> SYHKPDQQKLQALKDTANRLRISSIQATTAAGSGHPTSCCSAAEIMAVLFFHTMRYKSQDPRNPHNDRFVLSKGHAAPILYAVWAEAGFLAEAELLNLRKISSDLDGHPVPKQAFTDVATGSLGQGLGAACGMAYTGKYFDKASYRVYCLLGDGELSEGSVWEAMAFASIYKLDNLVAILDINRLGQSDPAPLQHQMDIYQKRCEAFGWHAIIVDGHSVEELCKAFGQAKHQPTAIIAKTFKGRGITGVEDKESWHGKPLPKNMAEQIIQEIYSQIQSKKKILATPPQEDAPSVDIANIRMPSLPSYKVGDKIATRKAYGQALAKLGHASDRIIALDGDTKNSTFSEIFKKEHPDRFIECYIAEQNMVSIAVGCATRNRTVPFCSTFAAFFTRAFDQIRMAAISESNINLCGSHCGVSIGEDGPSQMALEDLAMFRSVPTSTVFYPSDGVATEKAVELAANTKGICFIRTSRPENAIIYNNNEDFQVGQAKVVLKSKDDQVTVIGAGVTLHEALAAAELLKKEKINIRVLDPFTIKPLDRKLILDSARATKGRILT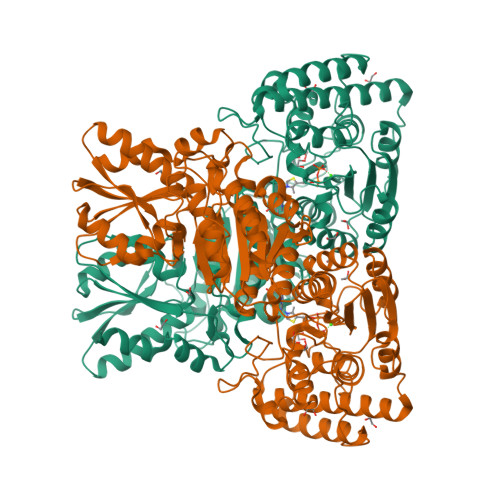VEDHYYEGGIGEAVSSAVVGEPGITVTHLAVNRVPRSGKPAELLKMFGIDRDAIAQAVRG>MGKEKTHINIVVIGHVDSGKSTTTGHLIYKCGGIDKRTIEKFEKEAAEMGKGSFKYAWVLDKLKAERERGITIDISLWKFETTKYYITIIDAPGHRDFIKNMITGTSQADCAVLIVAAGVGEFEAGISKNGQTREHALLAYTLGVKQLIVGVNKMDSTEPAYSEKRYDEIVKEVSAYIKKIGYNPATVPFVPISGWHGDNMLEPSPNMPWFKGWKVERKEGNASGVSLLEALDTILPPTRPTDKPLRLPLQDVYKIGGIGTVPVGRVETGILRPGMVVTFAPVNITTEVKSVEMHHEALSEALPGDNVGFNVKNVSVKDIRRGNVCGDSKSDPPQEAAQFTSQVIILNHPGQISAGYSPVIDCHTAHIACKFAELKEKIDRRSGKKLED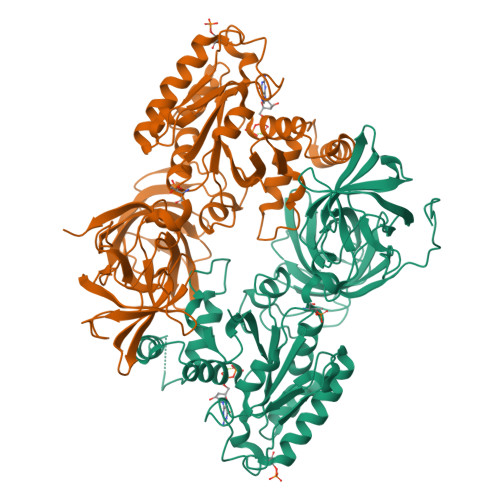NPKSLKSGDAAIVEMVPGKPMCVESFSQYPPLGRFAVRDMRQTVAVGVIKNVEKKSGGAGKVTKSAQKAQKAGK[2x]>[2x]MVRPSQSMYDRHLTIFSPDGNLYQIEYAIKAVKNTNITSVGVKGENCAVIISQKKMATQYISQDKLLDYNNITNIYNITDEIGCSMVGMPGDCLSMVYKARSEASEFLYSNGYNVNAETLCRNICDKIQVYTQHAYMRLHACSGMIIGIDENNKPELFKFDPSGFCAGYRACVIGNKEQESISVLERLLEKRKKKIQQETIDEDIRNTTILAIEALQTILAFDLKASEIEVAIVSTKNRNFTQISEKEIDNYLTYIAERD;>[2x]MADGEYSFSLTTFSPTGKLVQIEYALNRVSSSSPALGIRAKNGVIIATEKKSPNELIEENSIFKIQQISEHIGIVYAGMPGDFRVLLKRARKEAIRYSLQYGSEILVKELVKIIASIVQEFTQTGGVRPFGLSLLICGVDVYGYHLYQIDPSGCYFNWMATCVGKDYQNNMSFLEKRYNKDIEIEDAIHTAILTLKESYEGVLNEKNIEIGVAYDNKPFKILTQNEIKDYLIEIE;>MARRYDSRTTTFSPEGRLYQVEYALEAINNASITIGLITKDGVILGADKVFISKLIDKANNYEKIYKIDKHIFCGVAGLNADANILINQSRLYAQRYLYNYNEVQPVSQLVVQICDIKQSYTQYGGLRPYGVSFLIGGYDTKDGYQLYHTDPSGNYSGWFATAIGTNNLTASSVLKQEWKNDMTLEEGLLLALKTLAKSTDTEIPKSEKIELAYLTNKDGEVYQKYLTEKEIEELIKLYTQKYIKE[2x];>MSYDRAITVFSPDGHLLQVEHALEAVKKGGCAVAIKSSNFAVLAVEKKNIPKLQNPKTTEKLIKLDEHNCLAFAGLNADARVLVNKTRLECQRYYLNMDEPAPVDYIAKYVAKVQQKFTHRGGVRPFGIATLIAGFKNNKEICIYQTEPSGIYAAWKAQAIGKNAKIVQEFLEKNYQENMEQKDCIFLALKAIFEVVELSSKNVEVALLTEKDLTFIEEQEINSMVELIDQERTKNNEQNE[2x];>[2x]MFSTRSEYDRGVNTFSPEGRLFQVEYALGAIKLGSTAVGICVNDGVILASERRISSTLIEKDSVEKLLSIDDHIGCAMSGLMADARTLIDYARVECNHYKFIYNENINIKSCVELISELALDFSNLSDSKRKKIMSRPFGVALLIGGVDKNGPCLWYTEPSGTNTRFSAASIGSAQEGA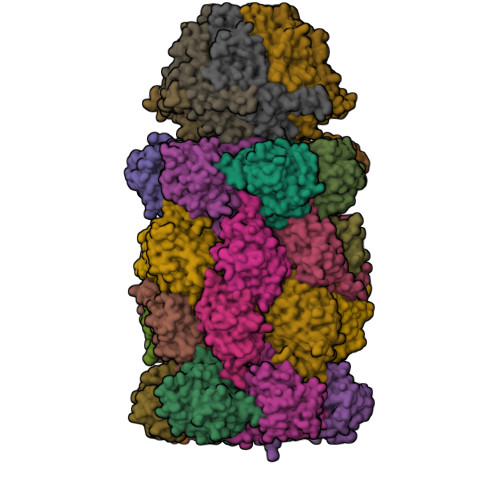ELLLQENYKKDMTFEQAEILALTVLRQVMEDKLSTSNVEICAIKKSDQTFYKYNTDDISRIIDVLPSPVYPTIDMTA;>[2x]MYRNLYDTDNIIYSPEGRLYQVEYASEAIKQGTCAVAIKSKDYVVVSGLKKCISKLSFPQEKIFKIDDYIGISMSGITSDAKVLTKFMQNECLSHKFLYNENINIESLVRSVADKYQKNTQKSSKRAFGVGLMIAAYHNEPCIFETRPNGSYFEYDALSFGARSHASKTYLEKNLHLFEECSLEELILHCLKALKCSLSSESELTISNTALAVVGKNHPWQEISSLQLEEYLSKVKMDAEQEQVEENVQNEANE;>MAGLSAGYDLSVSTFSPDGRLYQVEYIYKSINNNNTALCLECKDGIICCCINSNMDKNKMIKKNSYNRIYHVNNNIIITYSGFDGDARNIIDRARSEANTYYYNFHTNIPLHILVNRISLYIHAYTLYWHMRPFAASIIISSFNEKDKGDIYCIEPNGACYKYSGIVIGKNKEMFKTEIEKKDYKDINVRDAIEDIYKFILTSDDHMNKNNLQNLVNFSWICKESSYEFQNIHEEILTPALNKAVEYIEKLN[2x];>TTIIGIIYDNGVMLACDSRTSSGTFISNKCSRKINRINENLYVCRSGASAHSQKIIEIIKHYCVSMKNENRKKGRFHEGETIYDETTYDEEIDIDSINYLDYNNNNDNNLVTKNKYFYEDKFNDYNPLVENVAHITKKIIYTNNNFLSCALIFGGYDKIKKQQLYAVNLNGSIIEKHDFAVSGSGSIYIQSYLQDKYKKFMTKKECFNLILNCVKYAMHNDNSSGGLIRIVNITKSFVEEFTVVNTQMNFQY[2x];>TTICGLVCQNAVILGADTRATEGPIVADKNCSKLHYISKNIWCAGAGVAGDLEHTTLWLQHNVELHRLNTNTQPRVSMCVSRLTQELFKYQGYKVCAIVLGGVDVNGPQLYGIHPHGSSCLLPFTALGSGSLNAMAVLEAKYRDNMTIEEGKNLVCEAICAGIFNDLGSGGNVDICVITKDSYQHIRPYKEPNMRLYHLPHPTIYPKGTTPILSEKIEYIKKFISVEDA[2x];>[2x]MGSIYNYNGGCVLGMSGSNCVAIACDLRLGANTFTTVSTKFSKIFKMNNNVYVGLSGLATDIQTLYEILRYRVNLYEVRQDAEMDVECFANMLSSILYSNRFSPYFVNPIVVGFKLKHYVDEEGEKKVNYEPYLTAYDLIGAKCETRDFVVNGVTSEQLFGMCESLYVKDQDENGLFETISQCLLSALDRDCISGWGAEVLVLTPEKIIKKKLKARMD;>MDTLIGLRGNNFVVLAADTYSINSIIKLKNDDNTKFYDIHGNKCLLLGGSIGDRLQFGEFIRKNVHLYQYQNNTDMFVKSFAFFTRKNLAYYLRRNPFEVNCLIAGYDKKDGYQLYWCDYLSNMDSVNKGAHGYGAYLVSAILDKYYHENLTVDEALDIFKLCFEELKKRFLLTQINYELRIMYDNKVETQYVTV[2x];>[2x]TTTLAFKFKDGIIVAVDSRASMGSFISSQNVEKIIEINKNILGTMAGGAADCLYWEKYLGKIIKIYELRNNEKISVRAASTILSNILYQYKGYGLCCGIILSGYDHTGFNMFYVDDSGKKVEGNLFSCGSGSTYAYSILDSAYDYNLNLDQAVELARNAIYHATFRDGGSGGKVRVFHIHKNGYDKIIEGEDVFDLHYHYTNPEQKDQYVM;>[2x]MDLILYNDNLTEKKTEKENVIEHGRGFKRWYPYIDNGGTVIGLTGKDYVILAADTRLSLSYSIYTRFCPKISKLTDKCIIGSSGMQSDIKTLHSLLQKKIQLFVLEHSHYPDIHVIARLLCVILYSRRFFPYYAFNILAGVDENNKGVLYNYDSVGSYCEATHSCVGSGSQLILPILDNRVEQKNQLIKNTNFNLGDDINFVKDAITSATERDIYTGDKTLIYVIDKMGINVNTLDLKQD;>MTLGPVVTGTSVIAIKYKHGIMIAADRKASYGSYAKFQNVERIFKINNKTVMGFSGELADAQYLHELLTRKNINNLSEKKRKEDMYTPQHYHSYVSRVFYVRKNRIDPLFNNIIIAGINSQKYDNNDDNVLLYTNKNNDDEQNEYKNNEEYKEIHKDDLYIGFVDMHGTNFCDDYITTGYARYFALTLLRDHYKDNMTEEEARILINECLRILYFRDATSSNFIQIVKVTSKGVEYEEPYILPCVLNSADYVYPSTLLPPAGCMW[2x];>[7x]MEAYLNKIDKIEPSDQKIKEEYNKFKYDITKQAIESLRERIPKRIIFFNNLVNVNSEPGSILNVNDLDGVSYKYKINKIEENVRKKHKGNNSSDFDEREKKKDSLDGHVKHFSNNEDSKLIIDDKVLYTHYVPSHKQIYLELEKIKTYASELIEIIGNIKLWIQLNVPRIEDGNNFGVGIQEEAIQELARVEESAFNLYDAIVKYYMERAKISTKVLKYPNVSDYQEAVRELDEKEWIHIKITIVDMRNNYIMLYDLLYKNWEKVVKPKNEDAHHRMTF> AEVPLPQLRAYTVDASWLQPMAPLQIADHTWQIGTEDLTALLVQTPDGAVLLDGGMPQMASHLLDNMKARGVTPRD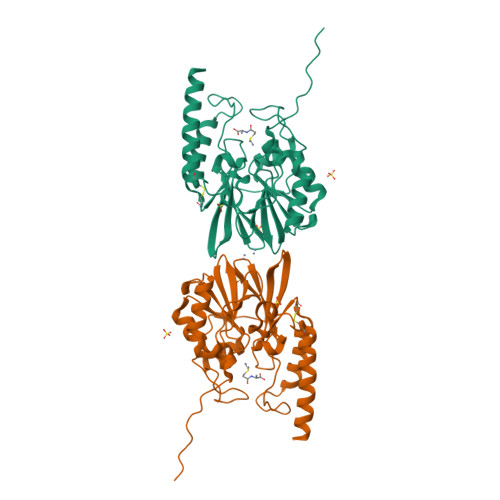LRLILLSHAHADHAGPVAELKRRTGAKVAANAESAVLLARGGSDDLHFGDGITYPPANADRIVMDGEVITVGGIVFTAHFMAGHTPGSTAWTWTDTRNGKPVRIAYADSLSAPGYQLQGNPRYPHLIEDYRRSFATVRALPCDVLLTPHPGASNWDYAAGARAGAKALTCKAYADAAEQKFDGQLAKETAGAR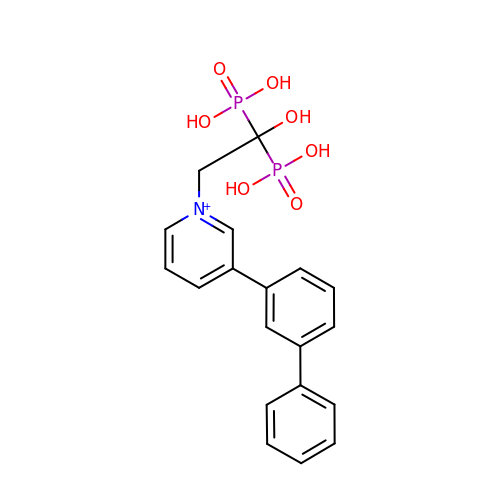3-BIPHENYL-3-YL-1-(2-HYDROXY-2,2-DIPHOSPHONOETHYL)PYRIDINIUM | C19 H20 N O7 P2 | SFGYQDTXSJEVCC-UHFFFAOYSA-O> APKAPA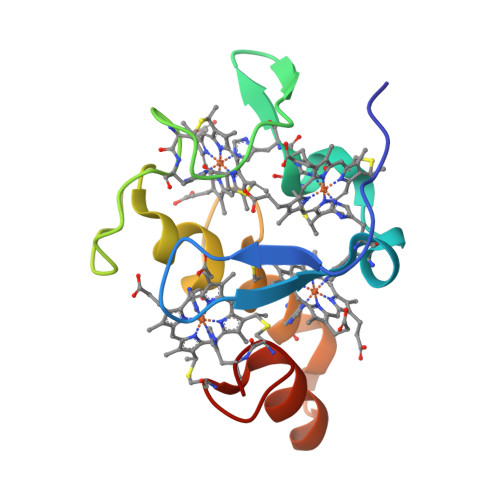DGLKMDKTKQPVVFNHSTHKAVKCGDCHHPVNGKEDYQKCATAGCHDNMDKKDKSAKGYYHAMHDKGTKFKSCVGCHLETAGADAAKKKELTGCKGSKCHS>RREQLMREEAEQKRLKTVLELQYVLDKLGDDEVRTDLKQGLNGVPILSEEELSLLDEFYKLVDPERDMSLRLNE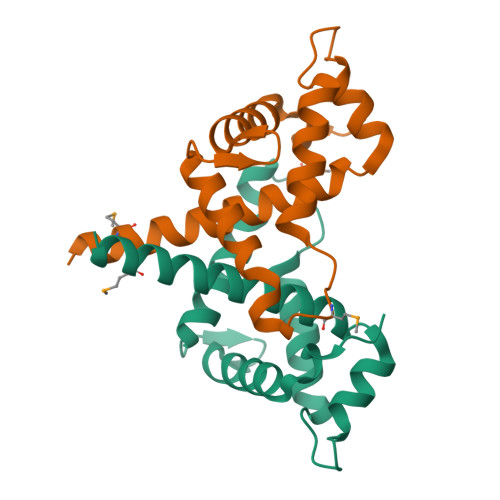QYEHASIHLWDLLEGKEKPVCGTTYKVLKEIVERVFQSNYFDSTHN[2x]(5~{R})-5-[(1~{R},3~{a}~{S},4~{E},7~{a}~{R})-7~{a}-methyl-4-[2-[(3~{R},5~{R})-4-methylidene-3,5-bis(oxidanyl)cyclohexylidene]ethylidene]-2,3,3~{a},5,6,7-hexahydro-1~{H}-inden-1-yl]-1-(4-hydroxyphenyl)hexan-1-one 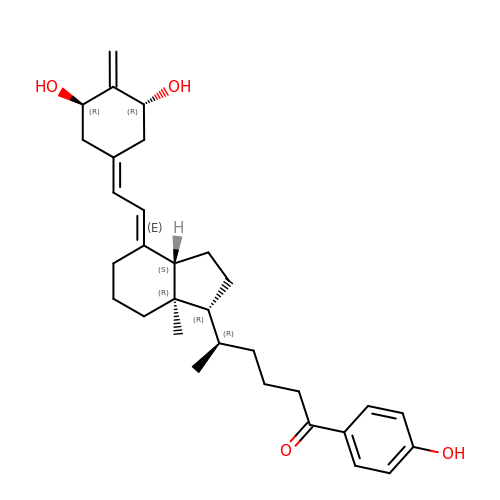| C31 H42 O4 | AVOJSQKILRAHNA-SLEIQBAPSA-N>[2x]GSHMRFDEFGNIITDSAVAEEPEPELPGVTEEALRLKEAALEELAAQEVTAPLVPLAVSAFLTSRKKAAAAELADWMQSPEGQASSLESIGRSLSRRNHGRSRAVVLAHDHDEAIKGLRAVAAGKQAPNVFSVDGPVTTGPVWVLAGFGAQHRKMGKSLYLRNEVFAAWIEKVDALVQDELGYSVLELILDDAQDYGIETTQVTIFAIQIALGELLRHHGAKPAAVIGQSLGEAASAYFAGGLSLRDATRAICSRSHLMGEGEAMLFGEYIRLMALVEYSADEIREVFSDFPDLEVCVYAAPTQTVIGGPPEQVDAILARAEAE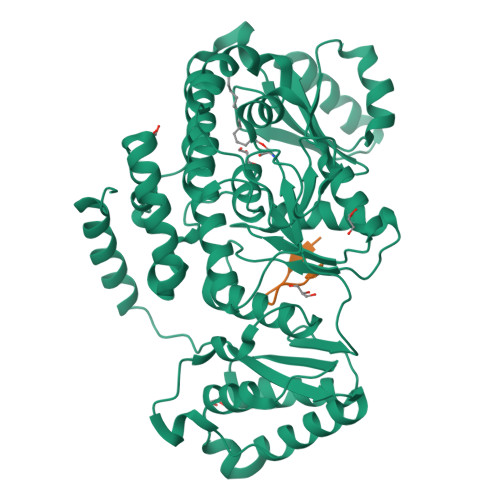GKFARKFATKGASHTSQMDPLLGELTAELQGIKPTSPTCGIFSTVHEGRYIKPGGEPIHDVEYWKKGLRHSVYFTHGIRNAVDSGHTTFLELAPNPVALMQVALTTADAGLHDAQLIPTLARKQDEVSSMVSTMAQLYVYGHDLDIRTLFSRASGPQDYANIPPTRF;>SDKENFWGMAVA[2x]>LYIQWL[2x]

Aggregation-prone-motifs (APRs) of proteins are short segments, which – as isolated peptides - form diverse amyloid-like crystals. We introduce two APRs - designed variants of the incretin mimetic Exendin-4 - that both display crystal-phase polymorphism. Crystallographic and spectroscopic analysis revealed that a single amino-acid substitution can greatly reduce topological variability: while LYIQWL can form both parallel and anti-parallel β-sheets, LYIQNL selects only the former. We found that a simple change in crystallization temperature or modest changes of chemical composition of the solvent system (therefore the available interaction partners) can prompt formation of significantly different nanostructures: we identified four different polymorphs of the LYIQWL and two of the LYIQNL APR peptides.

We previously characterized the APR of the Tc5b miniprotein – LYIQWL –, and found that it is able to form polymorphic amyloid crystal structures with both parallel and antiparallel β-sheets. To study the potential interference of TFA, we have lyophilized the peptide in HCl, and crystallized it again from 10 v/v% ethanol. Interestingly, crystals grown at 37 °C (in the absence of TFA) consisted of parallel β-sheets. In this case a simple temperature change lead to an anti-parallel/parallel switch: starting solutions of completely identical chemical composition resulted in amyloid-like crystalline phases of entirely different topology. On the other hand, in crystals from the present work, grown from a solution containing less ethanol and no residual TFA, neighbouring β-sheets run parallel to each other, resulting in two larger class 4 and two smaller class 1 interfaces leading to an overall class 4 topology. The hydrophobic residues (Leu1, Ile3, Trp5) form clusters in both structures, while hydrogen bonds are formed by chain termini, solvent molecules, Tyr2, Gln4 and Trp5 of chain A in the class 4 structure. A common structural feature in the two parallel LYIQWL structures is the presence of a weak Tyr – Tyr interaction. The geometric parameters characterising this interaction are similar in the two structures: the distance between the centres of the aromatic rings are 5.6 Å and 6.1 Å in the class 1 and class 4 structures, respectively, while the angle between the planes of the rings are 81.9° and 86.7°. In contrast to the class 1 structure, the class 4 structure did not contain ethanol molecules – only a water molecule could be identified in the electron density map. This suggests that the presence of an increased amount of ethanol is able to induce an anti-parallel to parallel reorientation of β-sheets, even without forming direct ethanol-peptide contacts within the amyloid nanostructure.>ADKLPYKVADIGLAAWGRKALDIAENEMPGLMRMREMYSASKPLKGARIAGCLHMTVETAVLIETLVALGAEVRWSSCNIFSTQDHAAAAIAKAGIPVFAWKGETDEEYLWCIEQTLHFKDGPLNMILDDGGDLTNLIHTKHPQLLSGIRGISEETTTGVHNLYKMMANGILKVPAINVNDSVTKSKFDNLYGCRESLIDGIKRATDVMIAGKVAVVAGYGDVGKGCAQALRGFGARVIITEIEPINALQAAMEGYEVTTMDEACKEGNIFVTTTGCVDIILGRHFEQMKDDAIVCNIGHFDVEIDVKWLNENAVEKVNIKPQVDRYLLKNGHRIILLAEGRLVNLGCAMGHPSFVMSNSFTNQVMAQIELWTHPDKYPVGVHFLPKKLDEAVAEAHLGKLNVKLTKLTEKQA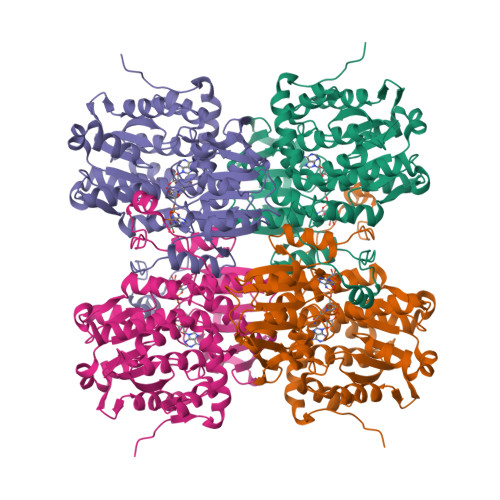QYLGMPINGPFKPDHYRY[4x]> MMAVSELEVDGVVFPSLARPPGSAHSHFLAGAGVRGMEIGGNFIKFTAIGVYLQADAAVSALAKKWAGKAADELASDAAFFRDVVTGEFEKFTQVTMILPLTGAQYSEKVTENCVAYWKAVGAYTDAEAAAVDKFKEAFKTETFPPGASILFTHSPAGVLTVAFSKNSSVPESGGAAIENRPLCEAVLEAIIGEHGVSPAAKLSLATRVAELLKEAASVDEPAAAEPVSVSA

In plants, flavonoid biosynthesis begins with phenylpropanoid metabolism in which phenylalanine is transformed into p-coumaroyl-coenzyme (Co)A. Chalcone synthase (EC 2.3.1.74), the first enzyme responsible for generating the basic flavonoid skeleton, then catalyzes the condensation of three molecules of malonyl-CoA with one molecule of p-coumaroyl-CoA to form chalcone. This is followed by the intramolecular and stereospecific cyclization of chalcone into (2S)-flavanone—a precursor of many downstream flavonoids—by chalcone-flavanone isomerase (CHI; EC 5.5.1.6). Type I CHIs—which are found in most plants including barley, rape, petunia, Arabidopsis, and rice—isomerize naringenin chalcone (2',4',6',4-tetrahydroxychalcone) into 5-hydroxy-flavonoid; whereas type II CHIs, common in leguminous plants, utilize both naringenin chalcone and isoliquiritigenin (2',4',4-trihydroxychalcone) to synthesize 5-deoxy-flavonoid. The family of genes encoding CHI in Deschampsia antartica—one of the only two vascular plant to naturally colonize the Maritime Antarctic—was recently characterized at the molecular level. The crystal structures of the unliganded and isoliquiritigenin-bound forms of DaCHI1 revealed that DaCHI1 can bind to type II substrates suggesting that DaCHI1 can produce antioxidant flavonoids from various substrates for protection against abiotic oxidative stresses.

The structures of unliganded DaCHI1 and the isoliquiritigenin-complexed catalytically inactive S189A mutant were determined at 2.7 and 2.1 Å resolution, respectively. Isoliquiritigenin-complexed DaCHI1 was crystallized in the P3221 space group with a single molecule in the asymmetric unit. An electron density map of isoliquiritigenin was observed near the entrance to the substrate-binding cleft. Isoliquiritigenin was bound via hydrophobic interactions with Met36, Ile38, Phe45, and Leu100. Notably, the 4'-hydroxyl group of isoliquiritigenin interacted directly with the NE atom of Arg34. The 4'-hydroxyl group of isoliquiritigenin also formed hydrogen bonds with Thr46 and Tyr105 mediated by two water molecules each. However, ligand binding caused an open/close movement around the strands of the β3–β4 region. However, isoliquiritigenin, which is a chalcone, exhibited a distinct mode of interaction, binding to the putative entrance of the hydrophobic binding pocket of DaCHI1. However, it should be noted that the S189A catalytic mutant protein was used to resolve the crystal structure of the DaCHI1-isoliquiritigenin complex; therefore, the isoliquiritigenin molecule could not go deep inside the substrate-binding pocket. As such, we cannot rule out the possibility that crystal packing inhibits the deep binding of isoliquiritigenin in the DaCHI1 active site.> GAMGSNPAEELAAAAQRGDVIAI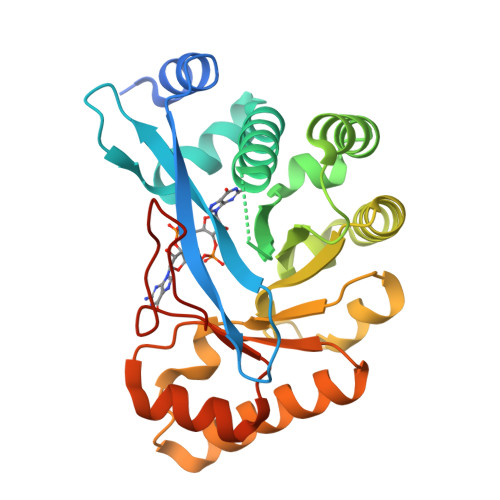LQQALETNSFRLLFQPVISLRGDSHENYEVLLRLLNPQGQEVPPAEFLHAAKEAGLAEKIDRWVILNSIKLLAEHRAKGHQTKLFVHLSSASLQDPGLLPWLGVALKAARLPPESLVFQISEADATSYLKQAKQLTQGLATLHCQAAISQFGCSLNPFNALKHLTVQFIKIDGSFVQDLNQVENQEILKGLIAELHEQQKLSIVPFVESASVLATLWQAGATYIQGYYLQGPSQAMDYDFSSGDE>[2x]MFSSMWRLPLWTLLALHRIHSAGAQDDVPPYFKTEPVRTQVHLEGNRLVLTCMAEGSWPLEFKWLHNNRELTRFSLEYRYMITSLDRTHAGFYRCIVRNRMGALLQRQTEVQVAYMGSFEEGEKRQSVNHGEAAVIRAPRISSFPRPQVTWFRDGRKIPPSSRIAITLENTLVILSTVAPDAGRYYVQAVNDKNGDNKTSQPITLAVENVGGPADPIAPTIIIP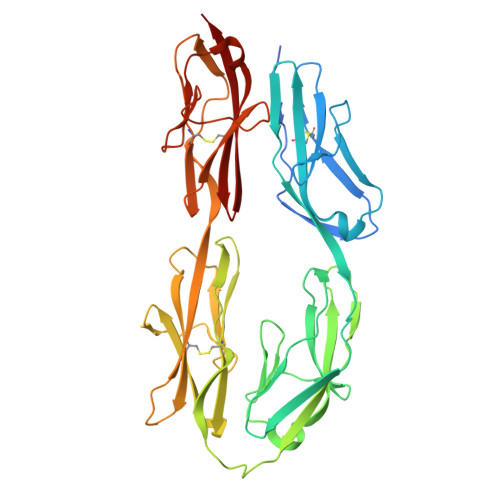PKNTSVVAGTSEVTMECVANARPLIKLHIVWKKDGAPLSSGISDYNRRLTIANPTVSDAGYYECEAMLRSSSVAPVTRGAYLSVLEPPQFVREPERHITAEMEKVVDIPCRAKGVPPPSITWYKDAALVEVGKLTRFKQRSDGGLQISGLLPDDTGMLQCFAHNAAGEAQTSTYLAVTS(3S,5S,7S)-tricyclo[3.3.1.1~3,7~]decan-1-amine | C10 H17 N | 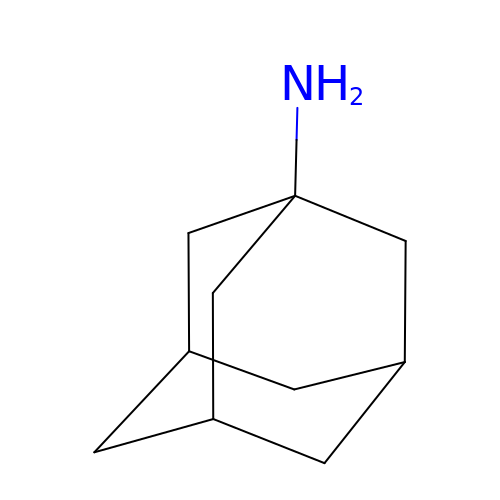DKNWSYNQZKUICI-CHIWXEEVSA-N>[4x]MTIFEKKPDFTLFLQTLSWEIDDQVGIEVRNELLRE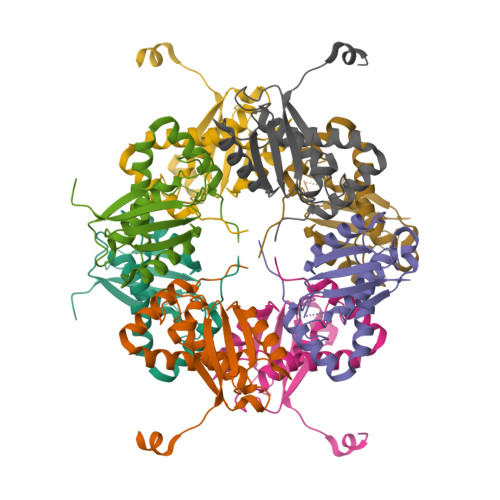VGRGMGTRIMPPPCQTVDKLQIELNALLALIGWGTVTLELLSEDQSLRIVHENLPQVGSAGEPSGTWLAPVLEGLYGRWVTSQAGAFGDYVVTRDVDAEDLNAVPRQTIIMYMRVRSSATHHHHHH> MSTQYETQGYTINNAGRRLVVDPITRIEGHMRCEVNINDQNVITNAVSCGTMFRGLEIILQGRDPRDAWAFVERICGVCTGVHALASVYAIEDAIGIKVPDNANIIRNIMLATLWCHDHLVHFYQLAGMDWIDVLDALKADPRKTSELAQSLSSWPKSSPGYFFDVQNRLKKFVEGGQLGIFRNGYWGHPQYKLPPEANLMGFAHYLEALDFQREIVKIHAVFGGKNPHPNWIVGGMPCAINIDESGAVGAVNMERLNLVQSIITRTADFINNVMIPDALAIGQFNKPWSEIGTGLSDKCVLSYGAFPDIANDFGEKSLLMPGGAVINGDFNNVLPVDLVDPQQVQEFVDHAWYRYPNDQVGRHPFDGITDPWYNPGDVKGSD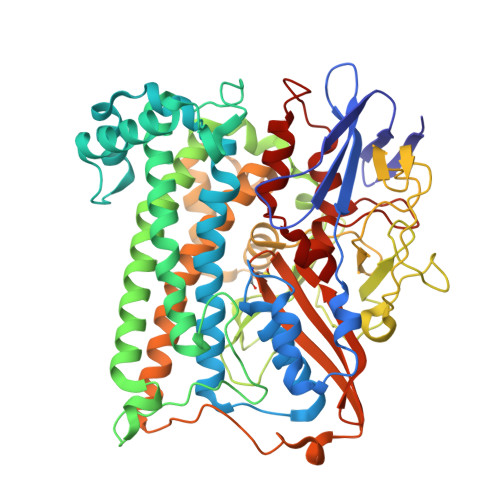TNIQQLNEQERYSWIKAPRWRGNAMEVGPLARTLIAYHKGDAATVESVDRMMSALNLPLSGIQSTLGRILCRAHEAQWAAGKLQYFFDKLMTNLKNGNLATASTEKWEPATWPTECRGVGFTEAPRGALGHWAAIRDGKIDLYQCVVPTTWNASPRDPKGQIGAYEAALMNTKMAIPEQPLEILRTLHSFNPCLACSTH>[8x]GKLPPYIFSPIPFLGHAIAFGKSPIEFLENAYEKYGPVFSFTMVGKTFTYLLGSDAAALLFNSKNED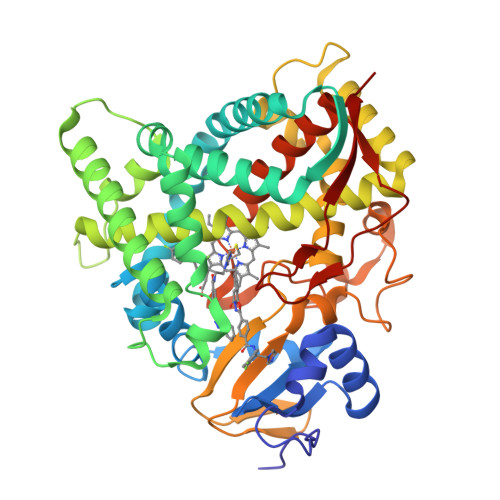LNAEDVYSRLTTPVFGKGVAYDVPNPVFLEQKKMLKSGLNIAHFKQHVSIIEKETKEYFESWGESGEKNVFEALSELIILTASHCLHGKEIRSQLNEKVAQLYADLDGGFSHAAWLLPGWLPLPSFRRRDRAHREIKDIFYKAIQKRRQSQEKIDDILQTLLDATYKDGRPLTDDEVAGMLIGLLLAGQHTSSTTSAWMGFFLARDKTLQKKCYLEQKTVCGENLPPLTYDQLKDLNLLDRCIKETLRLRPPIMIMMRMARTPQTVAGYTIPPGHQVCVSPTVNQRLKDSWVERLDFNPDRYLQDNPASGEKFAYVPFGAGRHRCIGENFAYVQIKTIWSTMLRLYEFDLIDGYFPTVNYTTMIHTPENPVIRYKRRSK> MRFKRGLVSCFIAILCLSVFLAGCSSNAKTGNEGSGSKGTKEGGVLTIARLSDADNLDPHFITNIPSASVVYHKVYENLVQRDKNMDFKPMLAKEWKQIDDLNWEFKLQQGVTFQDGAPFNAEAVKKNFERVLDPKVGSNRATVYSMIQEIKVIDEYTVQFILKYPYSPLLSIFASNEGSILSPKAIDEKGKGLAQHPVGTGPYTFKSWKPGEEIRLEKNKNYWGEKAKVDEVVFKVVPEDATRIGMIETSEAHIAENLPVTEVERVKNSPSMELIENEGLGVEYIGFNVEKKPFDNPLVRQAIAHAIETK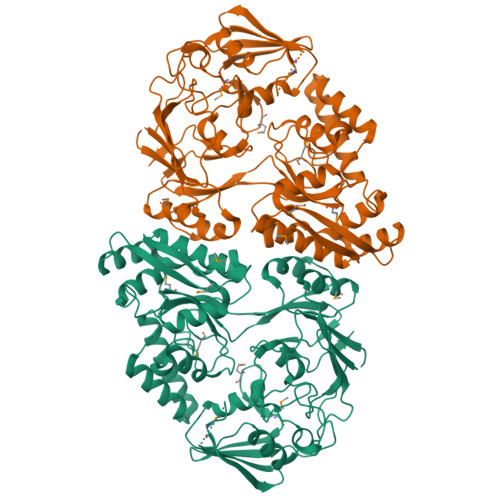GILKGVYNNVGTEINSVMTPKVFGYTKDVKGYKYDINTAKKLLADAGYPNGFKTTIWTNDSKVRMALVEVIQSQLKGIGVDVEIKVMEYGAFLAATNKSEHAMFVGGWGNATGDGDYNQYNLFHSSSHGATGNQFFYSNPEVDKLIEEARKEKDETKRKELYKQLQEIELKDALLVPIRGINHIAATTKNIKGFWIDPSGYLRLEGVELQ> GPEKTDEYLLARFKGDGVKYKAKLIGIDDVPDARGDKMSQDS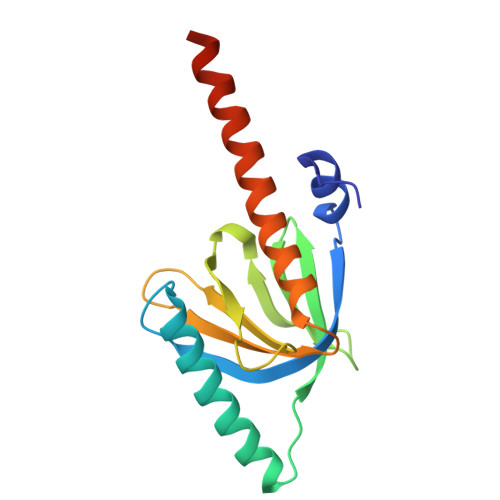MMKLKGMAAAGRSQGQHKQRIWVNISLSGIKIIDEKTGVIEHEHPVNKISFIARDVTDNRAFGYVCGGEGQHQFFAIKTGQQAEPLVVDLKDLFQVIYNVKKKEEEKKKIEEASKAVEN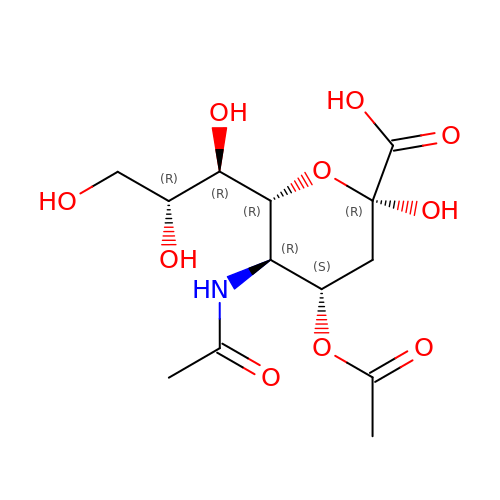4-O-acetyl-5-acetamido-3,5-dideoxy-D-glycero-alpha-D-galacto-non-2-ulopyranosonic acid | C13 H21 N O10 | LVBIMVQYUKOENY-CYBLFPARSA-N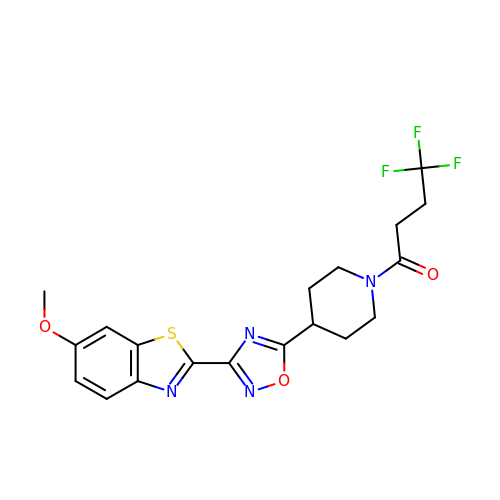4,4,4-tris(fluoranyl)-1-[4-[3-(6-methoxy-1,3-benzothiazol-2-yl)-1,2,4-oxadiazol-5-yl]piperidin-1-yl]butan-1-one | C19 H19 F3 N4 O3 S | MDFQKZXRTVTODM-UHFFFAOYSA-N> MLSSAHRAAFARPTATLWASARSFGAGPTRLLLGLEQVQDVPTSTDRKPTGMHRGPGKRQTAPKEAAQ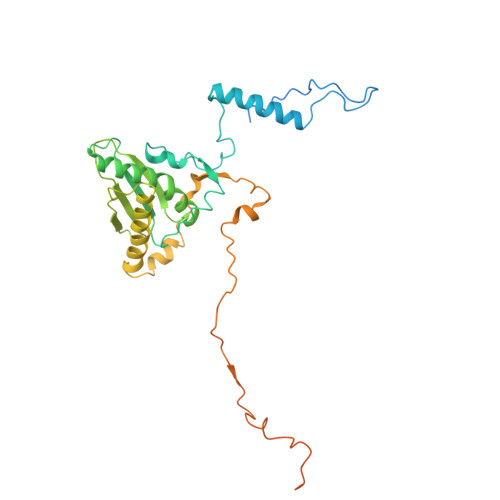YQFIKKWDLQMRETWDELEPFKGLPKPKVQFGNEAAEVIWPYALLLENVIKVHPYTKSIYVYYSQRQSTPLGELAARVAKRVSQAYLIPITFHNSHVYVEAEMLLEYSETPWVVVHCLDGTHKLIPVKPQAGQTVKEGAEEVLNGIVSACNEIGSAVKNPKEVMRLLSERPLQNQYVRVNYQWYGDTPEERMSHLVKWDYEPEEVVPQLRNRTQHVLDWMNYDGNLPTHNSVRVNIHREAARMRKPNVSAGPKTFFNSSGSRANARTARFDNSRSSQS>GHMATIHPTAIVDEGARIGAHSRIWHWVHICGGAEIGEGCSLGQNVFVGNRVRIGNRVKIQNNVSVYDNVFLEDDVFCGPSMVFTNVYNPRAAIERKSEYRDTIVRQGATLGANCTVVCGATIGRYAFVGAGAVVNKDVPDFAL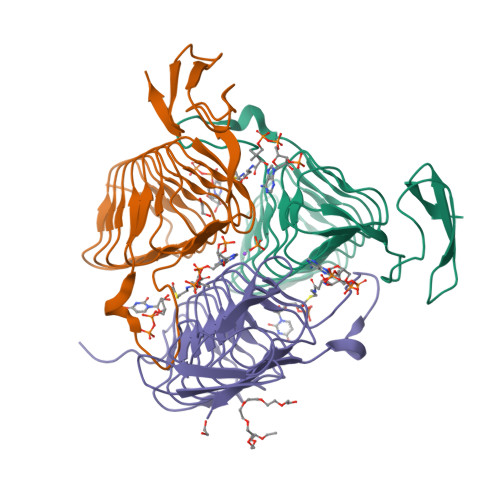VVGVPARQIGWMSRHGEQLDLPLRGNAEATCPHTGERYILTDGVCRLA[6x]> MDETGKALVLALYDYQEKSPREVTMKKGDILTLLNSTNKDWWKVEVNGRQGFVPAAYVKAL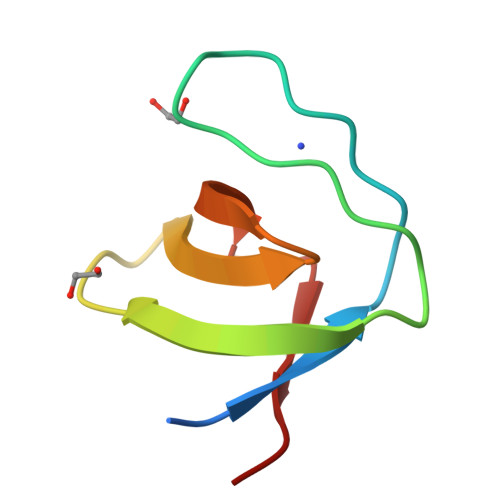D> MSDISQHYGGSLLAMIGKSSVAFLSDKRLGSGPISVSKNFTKIYSLTPRLFFGFTGLVSDGEMLFKKIRKNYNLFVQDNNKDMEPSELSNMISYILYQKRLQPYYVAVIVCGMTLDKKPYASSMDCIGAMKETSEFVTSGTASKNLMGLSEALFYPE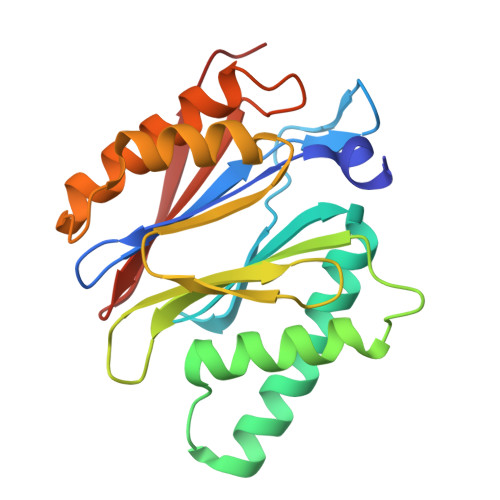MEDEDLFTTSVQTFLNSSDRDTFGGMGFECLLINPEGYKRREFVGRCD> MELKQAFVFEFDENLSSSSGSIHLEKVKQNCSPNYDYFKITFIDGYLYIKNKSGVILDKYDLKNVISLVALKRDYLSLSLSNN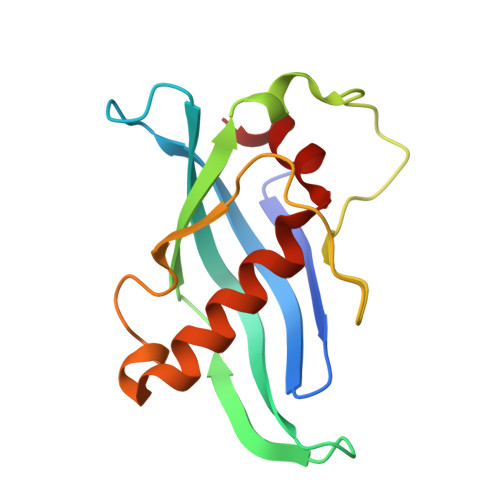KQIKKFKNIKNKHLKNKFNLYVINEDIEKRITKNGILEEVILNKMLLSILLGNEENLLQIS>MMLIKKIEELKNSEIKDIIDKRIQEFKSFKNKSNEEWFKELCFCILTANFTAEGGIRIQKEIGDGFLTLPREELEEKLKNLGHRFYRKRAEYIVLARRFKNIKDIVESFENEKVAREFLVRNIKGIGYQEASHFLRNVGYDDVAIIDRHILRELYENNYIDEIPKTLSRRKYLEIENILRDIGEEVNLKLSELDLYIWYLRTG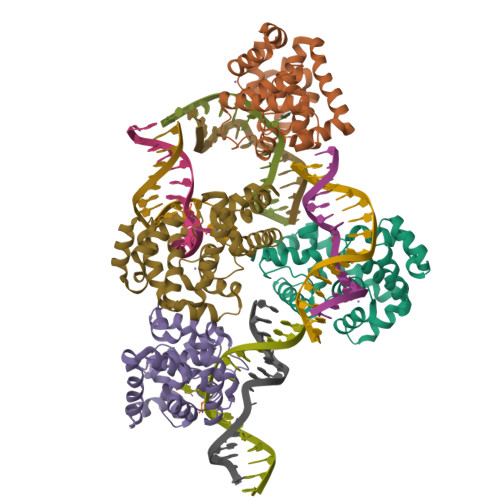KVLK[4x]>GSHMGSEDYKLREAQRELDKQRKDTEEI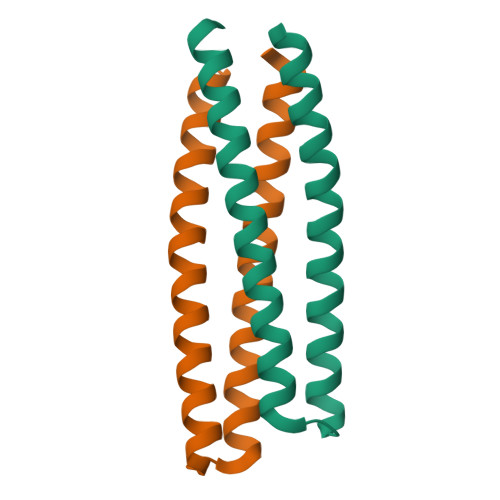RKRLKEIQRLTDERTSTADELIKELREIIRRLQEQSEKLREIIEELEKIIRKR[2x]>GPHMKRYNVITIFPEMINEIFKYGVLSKGIDIGLFRVNPINLRDYTEDKHKTVDDYQYGGGHGLVMKPEPIYKAIADLKSKKDTHVVFLDPRGEQFTQKTAERLYNYDDITFVCGRYEGIDDRVRELMADEMISIGDFVITGGELAAVTIIDAVARLIPGVLGDENSPNEESFTTGLLEYPHFTRPAEFMGKKVPEV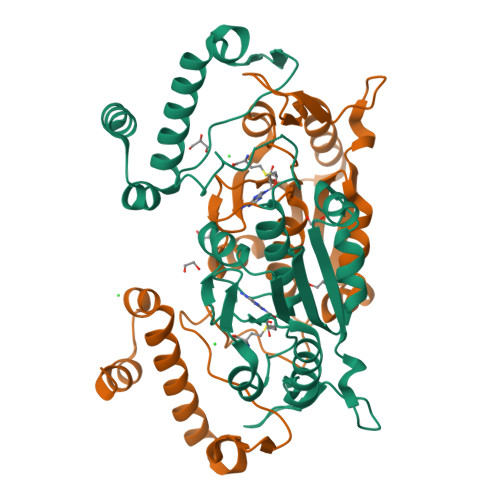LISGNHEEIRRWRLTESIKTTLQNRPDMILRKSLSREEEQILWSLT[2x]>[4x]MPPVGGKKAKKGILERLNAGEIVIGDGGFVFALEKRGYVKAGPWTPEAAVEHPEAVRQLHREFLRAGSNVMQTFTFYASEDKLENRGNYVLEKISGQEVNEAACDIARQVADEGDALVAGGVSQTPSYLSCKSETEVKKVFLQQLEVFMKKNVDFLIAEYFEHVEEAVWAVETLIASGKPVAATMCIGPEGDLHGVPPGECAVRLVKAGASIIGVNCHFDPTISLKTVKLM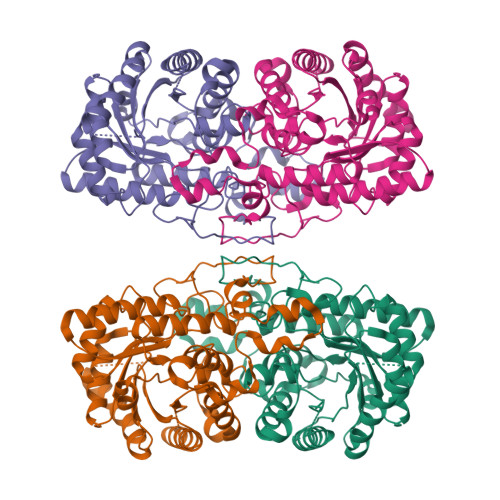KEGLEAARLKAHLMSQPLAYHTPDCNKQGFIDLPEFPFGLEPRVATRWDIQKYAREAYNLGVRYIGGCCGFEPYHIRAIAEELAPERGFLPPASEKHGSWGSGLDMHTKPWVRARARKEYWENLRIASGRPYNPSMSKPDGWGVTKGTAELMQQKEATTEQQLKELFEKQKFKSQ> GPDSMAMEMRLPVARKPLSERLGRDTKKHLVVPGDTITTDTGFMRGHGTYMGEEKLIASVAGSVERVNKLICVKALKTRYIGEVGDIVVGRITEVQQKRWKVETNS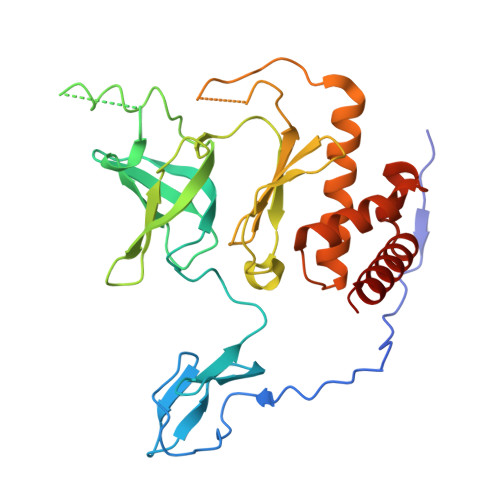RLDSVLLLSSMNLPGGELRRRSAEDELAMRGFLQEGDLISAEVQAVFSDGAVSLHTRSLKYGKLGQGVLVQVSPSLVKRQKTHFHDLPCGASVILGNNGFIWIYPTPEHKEEEAGGFIANLEPVSLADREVISRLRNCIISLVTQRMMLYDTSILYCYEASLPHQIKDILKPEIMEEIVMETRQRLLEQEG>[2x]MQKQAELYRGKAKTVYSTENPDLLVLEFRNDTSAGDGARIEQ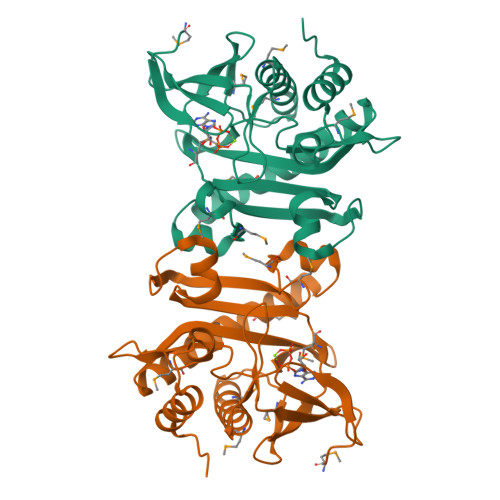FDRKGMVNNKFNYFIMSKLAEAGIPTQMERLLSDTECLVKKLDMVPVECVVRNRAAGSLVKRLGIEEGIELNPPLFDLFLKNDAMHDPMVNESYCETFGWVSKENLARMKELTYKANDVLKKLFDDAGLILVDFKLEFGLYKGEVVLGDEFSPDGSRLWDKETLEKMDKDRFRQSLGGLIEAYEAVARRLGVQLD> APAVADKADNAFMMICTALVLFMTIPGIALFYGGLIRGKNVLSMLTQVTVTFALVCILWVVYGYSLASGEGNNFFGNINWLMLKNIELTAVMGSIYQYIHVAFQGSFACITVGLIVGALAERIRFPAVLIFVVVWLTLSYIPIAHMVWGGGLLASHGALDFAGGTVVHINAAIAGLVGAYLIGKRVGFGKEAFKPHNLPMVFTGTAILYIGWFGFNAGSAGTANEIAALAFVNTVVATAAAILGWIFGEWALRGLPSLLGACSGAIAGLVGVTPACGYIGVGGALIIGVVAGLAG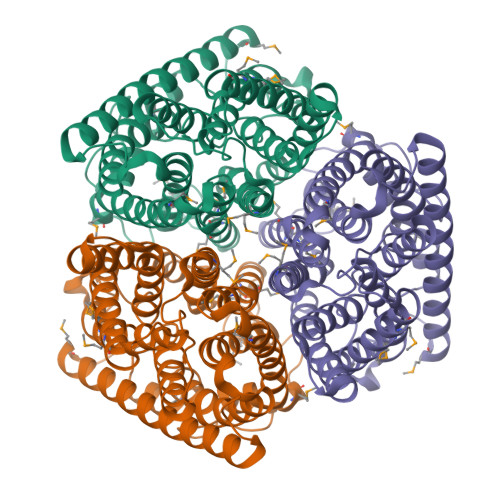LWGVTMLKRLLRVDDPCDVFGVHGVCGIVGCIMTGIFAASSLGGVGFAEGVTMGHQLLVQLESIAITIVWSGVVAFIGYKLADLTVGLRV> GLIVDTRDVEERVHVMRKTELAPTVAHGVFNPEFGPAALSNKDPRLNEGVVLDEVIFSKHKGDTKMSAEDKALFRRCAADYASRLHSVLGTANAPLSIYEAIKGVDGLDAMEPDTAPGLPWALQGKRRGALIDFENGTVGPEVEAALKLMEKREYKFACQTFLKDEIRPMEKVRAGKTRIVDVLPVEHILYTRMMIGRFCAQMHSNNGPQIGSAVGCNPDVDWQRFGTHFAQYRNVWDVDYSAFDANHCSDAMNIMFEEVFRTEFGFHPNAEWILKTLVNTEHAYENKRITVEGGMPSG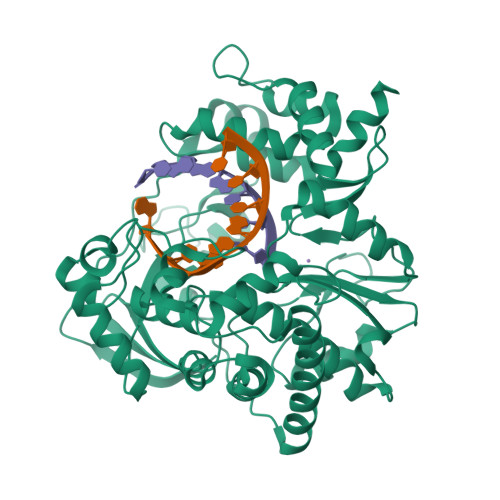CSATSIINTILNNIYVLYALRRHYEGVELDTYTMISYGDDIVVASDYDLDFEALKPHFKSLGQTITPADKSDKGFVLGHSITDVTFLKRHFHMDYGTGFYKPVMASKTLEAILSFARRGTIQEKLISVAGLAVHSGPDEYRRLFEPFQGLFEIPSYRSLYLRWVNAVCGDAAALEHHHHHHH> MNINQLILRNLKKNLRNYYLYVFALIFSVALYFAFVTLQYDPAINEVKASIKGAAAIKTASILLVAVVAIFILYANTIFIKRRSKEIGLFQLIGMTKHKIFRILSAENVMLYFGSLAIGVAAGFSISKLVLMILFKIVDVKADAKLHFSEQALVQTVIVFCGIYLLIMIMNYTFIKKQSILSLFKVTSSTEDKVKKISFFQMLIGALGIVLILTGYYVSSELFGGKFKTINELFVAMSFILGSVIIGTFLFYKGSVTFISNIIRKSKGGYLNISEVLSLSSIMFRMKSNALLLTIITTVSALAIGLLSLAYISYYSSEKTAEQNVAADFSFMNEKDAKLFENKLRESNISFVKKATPVLQANVDIANIMDGTPKEMQGDPGNMQLAVVSDKDVKGVDVAAGEAVFSGYTDLLQKIMVFKDSGVIKVKSKHETQPLKYKGLREEFLVSYTFTSGGMP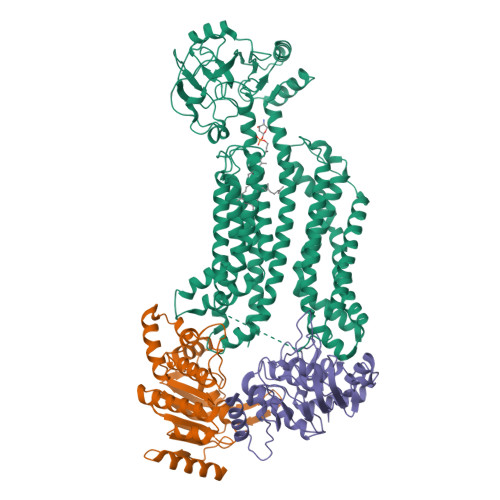AVIVDDSLFKQLDKDKDPRIQLAQSTFIGVNVKHDDQMEKANELFQQVNKKNEHLSRLDTSAAQKSLFGMVMFIVGFLGLTFLITSGCILYFKQMGESEDEKPSYTILRKLGFTQGDLIKGIRIKQMYNFGIPLVVGLFHSYFAVQSGWFLFGSEVWAPMIMVMVLYTALYSIFGFLSVLYYKKVIKSSL;>[2x]MSGHHHHHHVILEANKIRKSYGNKLNKQEVLKGIDIHIEKGEFVSIMGASGSGKTTLLNVLSSIDQVSHGTIHINGNDMTAMKEKQLAEFRKQHLGFIFQDYNLLDTLTVKENILLPLSITKLSKKEANRKFEEVAKELGIYELRDKYPNEISGGQKQRTSAGRAFIHDPSIIFADEPTGALDSKSASDLLNKLSQLNQKRNATIIMVTHDPVAASYCGRVIFIKDGQMYTQLNKGGQDRQTFFQDIMKTQGVLGGVQHEH> MHHHHHHHHHHGENLTFQGMKKYKKFCFLGIGLLPLVLASCGTNTATKDSQDATEKKVEQVATLTAGTPVQSLDPATAVDQTSITLLANVMEGLYRLDEKNQPQPAIAAGQPKVSNNGKTYTIVIRDGAKWSDGTQITASDFVAAWQRVVDPKTVSPNVELFSAIKNAKEIASGKQAKDTLAVKSIGEKTLEIELVEPTPYFTDLLSLTAYYPVQQKAIKEYGKDYGVSQKAIVTNGAFNLTNLEGVGTSDKWTISKNKEYWDQKDVSMDKINFQVVKEINTGINLYNDGQLD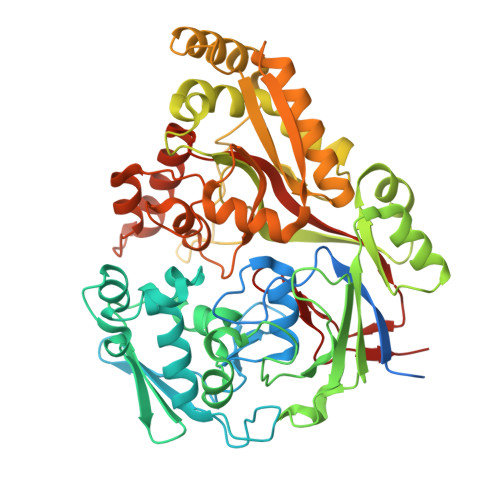EAPLAGEYAKQYKKDKEYSTTLMANTMFLEMNQTGENKLLQNKNVRKAINYAIDRESLVKKLLDNGSVASVGVVPKEMAFNPVNKKDFANEKLVEFNKKQAEEYWDKAKKEIDLSKNTSLDLLVSDGEFEKKAGEFLQGQLQDSLEGLKVTVTPIPANVFMERLTKKDFTLSLSGWQADYADPISFLANFETNSPMNHGGYSNKNYDELLKDSSSKRWQELKKAEKLLINDMGVVPIFQVGTAKLEKSKIKNVLMHSIGAKYDYKKMRIEK~{N}-[(1-pyridin-2-ylpiperidin-4-yl)methyl]pyrrolidine-1-carboxamide | C16 H24 N4 O | 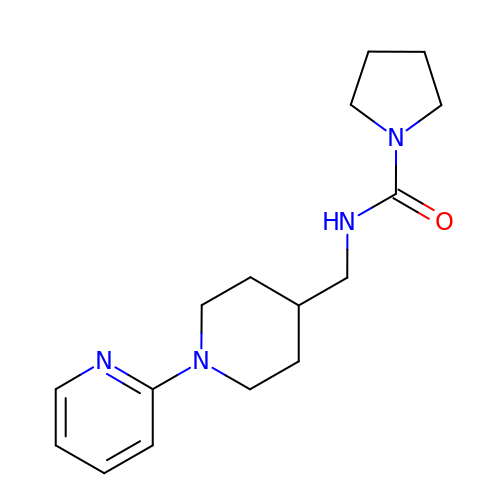FCULEXINIXPVIT-UHFFFAOYSA-N>XSLSDKDKAAVRALWSKIGKSSDAIGNDALSRMIVVYPQTKIYFSHWPDVTPGSPNIKAHGKKVMGGIALAVSKIDDLKTGLMELSEQHAYKLRVDPSNFKILNHCILVVISTMFPKEFTPEAHVSLDKFLSGVALALAERYR[2x];>[2x]VEWTDKERSIISDIFSHMDYD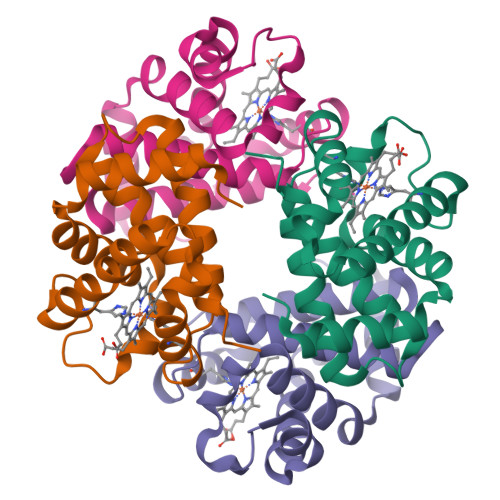DIGPKALSRCLVVYPWTQRYFSGFGNLYNAEGIMSNANVAAHGIKVLHGLDRGMKNMDNIADAYTDLSTLHSEKLHVDPDNFKLLSDCITIVLAAKMGHAFTAETQGAFQKFLAAVVSALGKQYH>MNLIPTVIETTNRGERAYDIYSRLLKDRIIMLGSQIDDNVANSIVSQLLFLQAQDSEKDIYLYINSPGGSVTAGFAIYDTIQHIKPDVQTICIGMAAAMGSFLLAAGAKGKRFALPNAEVMIHQPLGGAQGQATEIEIAANHILKTREKLNRILSERTGQSIEKIQKDTDRDNFLTAEEAKEYGLIDEV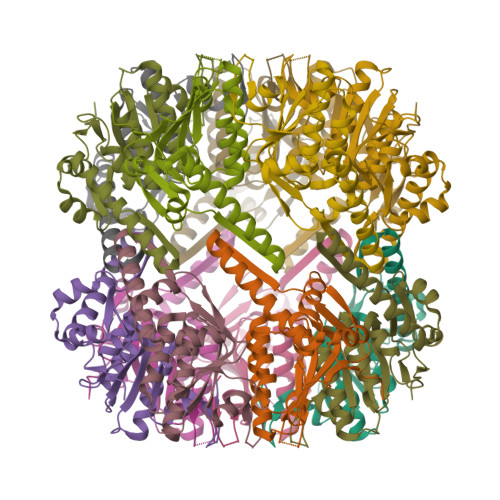MVPETKWSHPQFEK[28x]> GPR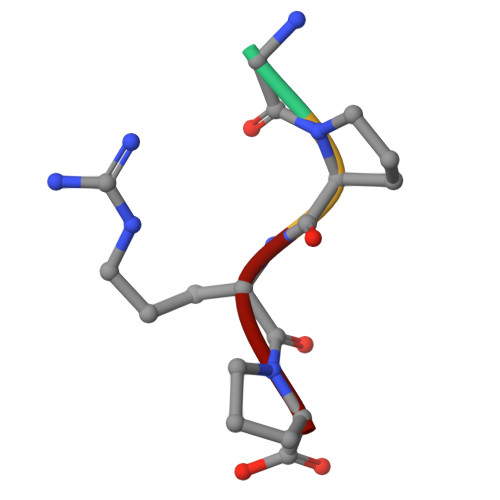P>[2x]MSLSTGATIVIDLGKTLSKVSLWDLDGRMLDRQVRPSIPLEIDGIRRLDAPDTGRWLLDVLSRYADHPVTTIVPVGHGAGIAALTDGRLAFPPLDYEQSIPEAVMADYRSQRDPFARTGSPALPDGLNIGSQLWWLDQLHPDVMANATLLPWAQYWAWFLTGRAVSEVTSLGCHSDLWDPQDGDFSPMAKRLGWAAR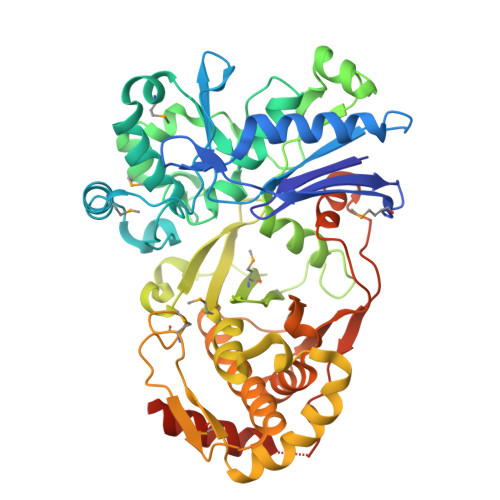FAPIVRAGDTVGALLPAIAERTGLSPDVQVLAGLHDSNAALLAARGFAEIADNEATVLSTGTWFIAMRLPATPVDTATLPEARDCLVNVDVHGRPVPSARFMGGREIETLIEIDTRRVDIKPDQPALLAAVPEVLRHGRMILPTLMRGFGPYPHGRFAWINRPEDWFERRAAACLYAALVADTALDLIGSTGRILVEGRFAEADVFVRALASLRPDCAVYTANAHNDVSFGALRLIDPGLRPQGELVRIEPLDTGSWADLDTYRNRWQAEVEAAKVEEGHHHHHH>[2x]MRGSGSMDSSVIQRKKVAVIGGGLVGSLQACFLAKRNFQIDVYEAREDTRVATFTRGRSINLALSHRGRQALKAVGLEDQIVSQGIPMRARMIHSLSGKKSAIPYGTKSQYILSVSRENLNKDLLTAAEKYPNVKMHFNHRLLKCNPEEGMITVLGSDKVPKDVTCDLIVGCDGAYSTVRSHLMKKPRFDYSQQY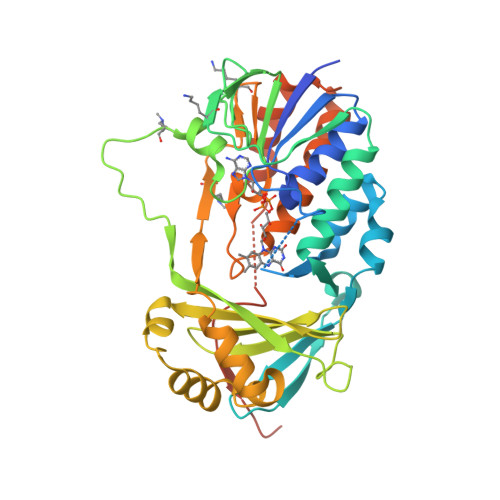IPHGYMELTIPPKNGDYAMEPNYLHIWPRNTFMMIALPNMNKSFTCTLFMPFEEFEKLLTSNDVVDFFQKYFPDAIPLIGEKLLVQDFFLLPAQPMISVKCSSFHFKSHCVLLGDAAHAIVPFFGQGMNAGFEDCLVFDELMDKFSNDLSLCLPVFSRLRIPDDHAISDLSMYNYIEMRAHVNSSAAALEHHHHHH>[2x]MSLANKPLAKALETISGIPITPFRKSDGSIDWHHYKETVDRIVDNGIDVIVPCGNTSEFYALSLEEAKEEVRRTVEYVHGRALVVAGIGYATSTAIELGNAAKAAGADAVMIHMPIHPYVTAGGVYAYFRDIIEALDFPSLVY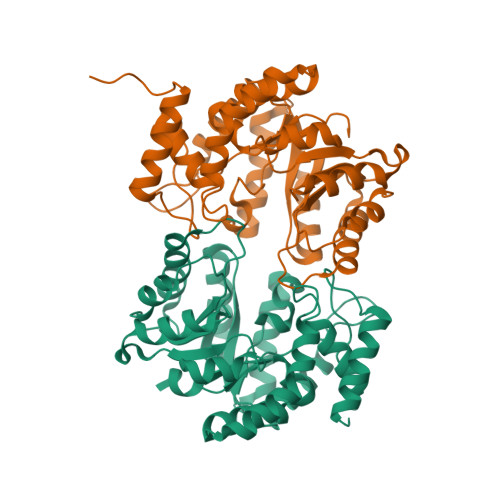FKDPEISDRVLVDLAPLQNLVGVKYAINDLPRFAKVVRSIPEEHQIAWICGTAEKWAPFFWHAGAKGFTSGLVNLLPQKAVEMLEALRNNDNDAVWRIWEDIVPFEDLRGKYNQGNNVVVIKEAMEMLRQNAGVTRAPVNELSNEDKQLVTELLSSWKLLQPTKGEGHHHHHH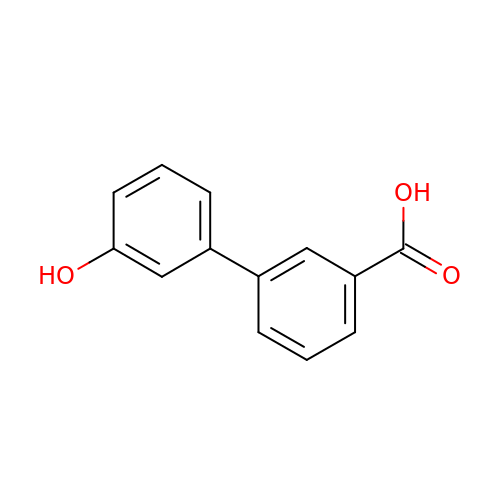3-(3-hydroxyphenyl)benzoic acid | C13 H10 O3 | CTFCUBMVYRSJLK-UHFFFAOYSA-N> MTIRRPEHFTHHEVQLSDVKIHYVREGAGPTLLLLHGWPGFWWEWSKVIGPLSERFDVIVPDLRGFGDSEKPDLSDLAQYSLERVADDQAELLNALGIDQAYVVGHDYSAIVVHKFIRKYPDRVVKAAIFDPITPDFGPFYLGFPHIAESWYSQFHQTDMSVELVTSSREACRIYFKHFFDHWSYHAPLLTQDELDIYVDNCMKPNNVHGGFNYYRSNLSVTSDPWTDLDRTVSDLPVTMLWGVGDPVVPSSLVHQVPNYYSN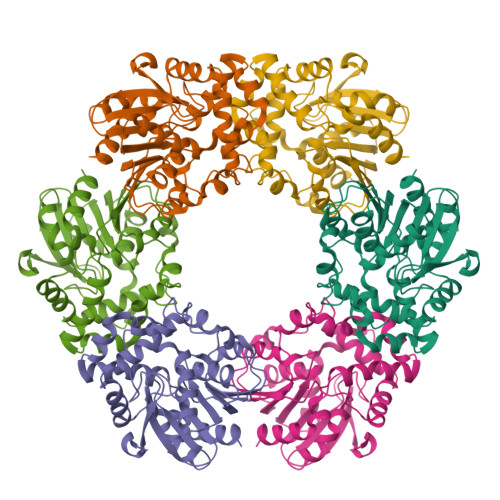YTMELIQDAGHFMMVEKPEVVIDRLKAGFR> GGGHMSKVFAVYGASGCGRSLMPVANEQLRILEGDTDSQIVFIDDALDDNITVNGYTAMNYTKFKSIKNDDKFVLI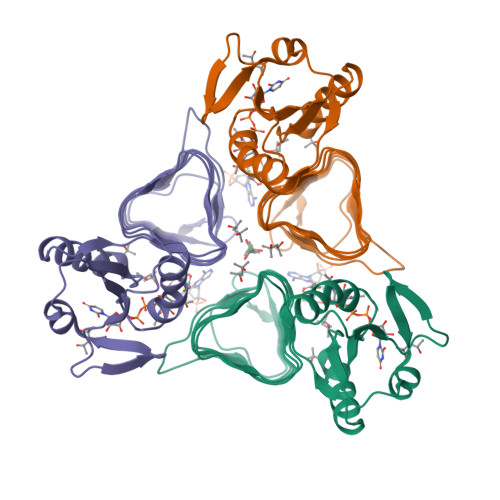AIANSSIRQKIADKLVKDGISLWTVQGMTTLIMDEVSIDAGAALSPFVTIAANVTIGKCFHANLYSYVEHDCIIGDYVTFAPRVSCNGNIHIHDHAYIGTGAVIKQGTPDKPLIIGKGAIVGMGAVVTKEVPAGAVVIGNPARLLNK>[2x]MGGFSQSCLPNWIMHGKSCYLFSFSGNSWYGSKRHCSQLGAHLLKIDNSKEFEFIESQTSSHRINAFWIGLSRNQSEGPWFWEDGSAFFPNSFQVRNAVP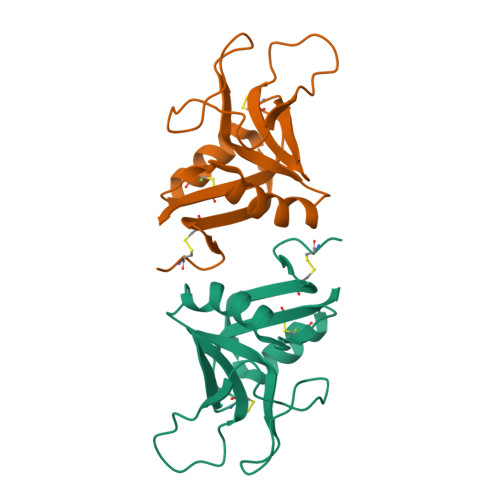QESLLHNCVWIHGSEVYNQICNTSSYSICEKELKHHHHHH> DYKDDDDKAAAVDFPWAAVDNMMVRKGDTAVLRCYLEDGASKGAWLNRSSIIFAGGDKWSVDPRVSISTLNKRDYSLQIQNVDVTDDGPYTCSVQTQHTPRTMQVHL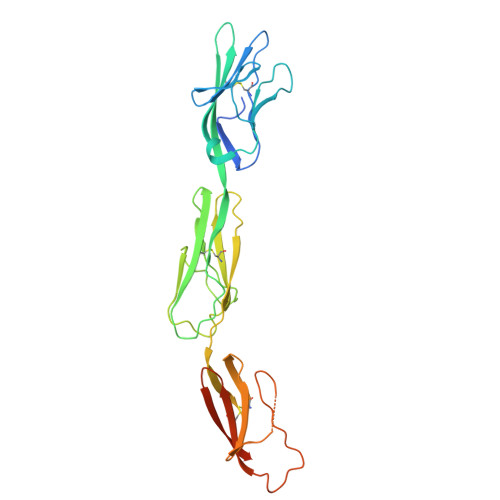TVQVPPKIYDISNDMTVNEGTNVTLTCLATGKPEPSISWRHISPSAKPFENGQYLDIYGITRDQAGEYECSAENDVSFPDVRKVKVVVNFAPTIQEIKSGTVTPGRSGLIRCEGAGVPPPAFEWYKGEKKLFNGQQGIIIQNFSTRSILTVTNVTQEHFGNYTCVAANKLGTTNASLPLNPPSTAQYGITGLEVLFQ> MEFRMKVFKDVFTNDEVCSDSYVQQDPFEVPEFREIAFEVKS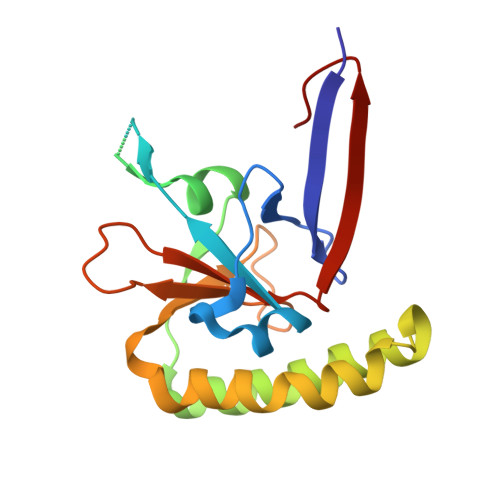NKRIKGNEDYGIADNSEDAVEGMGADVEHVIDIVDSFQLTSTAFSKKEYSAYIKNYMQKVAKYLEEKKPDRVEIFKTKAQPFIKHILTNFDDFEFYMGESLDMEAGIIYSYYKGEEITPRFVYISDGLFEEKYLEHHHHHH>SSTQIGGMSLDQARTQLAPWTQRAAPIGADEYQQRIERARVLMRAQGVDALLIGAGTSLRYFSGVPWGASERLVALLLTTEGDPVLICPAFEEGSLDAVLQLPVRKRLWEEHEDPYALVVQAMDEQHAHALALDPGIAFA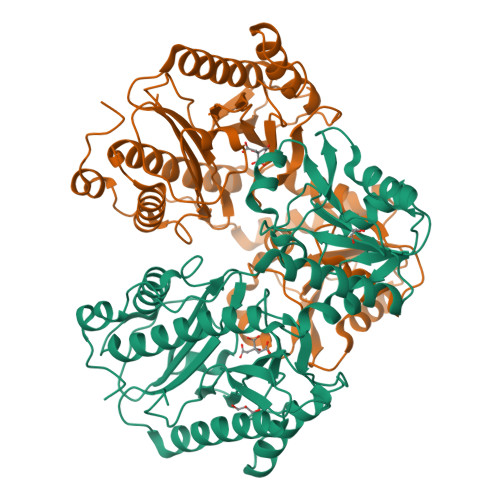VHTGLRAHLGTAIRDAGAIIDGCRMCKSPAELALMQQACDMTLLVQRLAAGIAHEGIGTDQLVRFIDEAHRALGADNGSTFCIVQFGHATAFPHGIPGVQHLRAGELVLIDTGCTVQGYHSDITRTWIYGTPSDAQQRIWELELAAQAAAFAAVRPGVACEAVDQAARAVLQAAGLGPDYRLPGLPHRTGHGCGLAIHEAPYLVRGNRQPLQPGMCASNEPMIVVPGAFGVRLEDHFYVTDTGAQWFTPPSVAIDQPFA[2x]> MVTVVEEVDHLPIYDLDPKLEEFKDHFNYRIKRYLDQKCLIEKHEGGLEEFSKGYLKFGINTVDGATIYREWAPAAQEAQLIGEFNNWNGAKHKMEKDKFGIWSIKISHVNGKPAIPHNSKVKFRFRHGGGAWVDRIPAWIRYATFDASKFGAPYDGVHWDPPACERYVFKHPRPPKPDAPRIYEAHVGMSGEEPEVSTYREFADNVLPRIRANNYNTVQLMAIMEHSYYASFGYHVTNFFAVSSRSGTPEDLKYLVDKAHSLGLRVLMDVVHSHASNNVTDGLNGYDVGQNTHESYFHTGDRGYHKLWDSRLFNYANWEVLRFLLSNLRYWMDEFMFDGFRFDGVTSMLY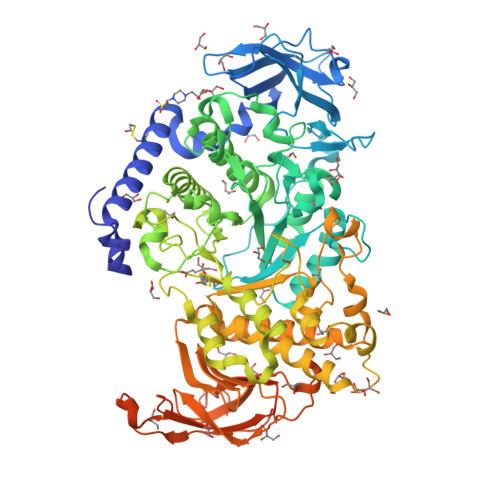HHHGINKGFTGNYKEYFSLDTDVDAIVYMMLANHLMHKLLPEATIVAEDVSGMPVLCRPVDEGGVGFDFRLAMAIPDRWIDYLKNKEDRKWSMSEIVQTLTNRRYTEKCIAYAESHDQSIVGDKTIAFLLMDKEMYTGMSDLQPASPTINRGIALQKMIHFITMALGGDGYLNFMGNEFGHPEWIDFPREGNNWSYDKCRRQWSLVDTDHLRYKYMNAFDQAMNALEEEFSFLSSSKQIVSDMNEKDKVIVFERGDLVFVFNFHPNKTYKGYKVGCDLPGKYRVALDSDALVFGGHGRVGHDVDHFTSPEGMPGVPETNFNNRPNSFKVLSPPRTCVAYYRVDEDREELRRGGAVASGKIVTEYIDVEATSGETISGGWKGSEKDDCGKKGMKFVFRSSDEDCK> GDPNQAVLKFTTEIHPSCVTRQKVIGAGEFGEVYKGMLKTSSGKKEVPVAIKTLKAGYTEKQRVDFLGEAGIMGQFSHHNIIRLEGVISKYKPMMIITEYMENGALDKFLREKDGEFSVLQLVGMLRGIAAGMKYLANMNYVHRDLAARNILVNSNLVCKVSDFGLSRVLEDDPEATY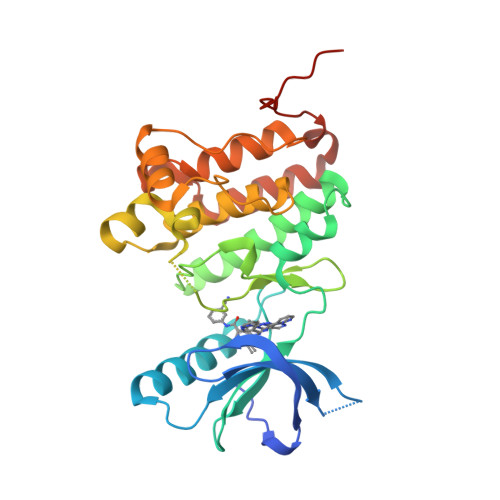TTSGGKIPIRWTAPEAISYRKFTSASDVWSFGIVMWEVMTYGERPYWELSNHEVMKAINDGFRLPTPMDCPSAIYQLMMQCWQQERARRPKFADIVSILDKLIRAPDSLKTLADFDPRVSIRLPSTSG In the present study, we elucidated the crystal structure of Mycobacterium tuberculosis H37Rv HigA2 (hereafter referred to as MtHigA2), which contains an HTH motif. The HigA antitoxin represses the transcription of HigBA or forms a stable HigBA complex, thereby preventing the ribonuclease activity of the HigB toxin and the associated cytotoxic events. Structural studies of MtHigA2 confirmed that it has three regions: (i) a disordered N-terminus that is liable to cleavage, (ii) an α-helix bundle containing an HTH motif for DNA binding and (iii) a β-lid for dimerization. The antitoxin MtHigA2 has two binding partners: DNA and the toxin MtHigB2.

The crystal structure of MtHigA2 was determined from three distinct crystal forms. Form I belonged to space group P212121 and was determined to 2.0 Å resolution, form II packed in space group P43212 and was determined to 3.2 Å resolution, and form III was solved in space group P3121 to 3.4 Å resolution. However, the N-terminal ∼25 residues are unstructured in all three observed crystal forms. All dimers share the β-lid as their major dimeric interface, but the position of the α-helix bundle varies. When the different dimers are aligned based on a single HTH motif from one monomer, the corresponding motif in the dimer pair shows a different relative position. The flexibility in dimerization leads to drastic changes in the locations of positively charged residues on the HTH motif, including His54, Arg56 and Arg59. To predict the physiological dimer, each form was submitted to the PISA server to calculate the strength of the dimer interface. Interestingly, all of the forms had similarly favourable dissociation energies (ΔG): −14, −15 and −17 kcal mol−1 for forms I, II and III, respectively. This suggests that the flexibility of the β-lid does not impact the formation of a stable dimer and is likely to contribute to function. The three different crystal structures in our study reveal the flexibility in dimerization mode while anchored by the β-lid.

>[5x]MAMTLRDMDAVRPVNREAVDRHKARMRDEVRAFRLRELRAAQSLTQVQVAALAHIRQSRVSSIENGDIGSAQVNTLRKYVSALGGELDITVRLGDETFTLA> KETAAAKFERQHMDSSTS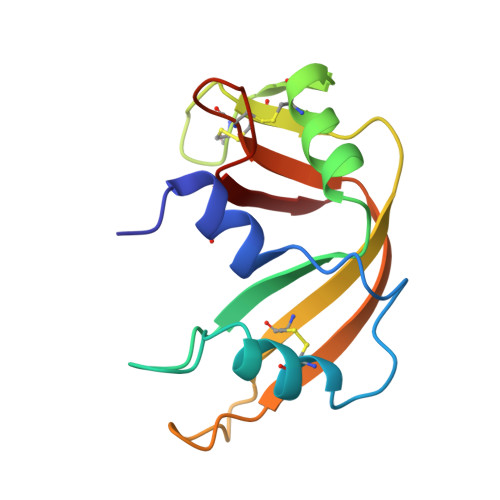AASSSNYCNQMMKSRNLTKDRAKPVNTFVHESLADVQAVCSQKNVACKNGQTNCYQSYSTMSITDCRETGSSKYPNAAYKTTQANKHIIVACEGNPYVPVHFDASV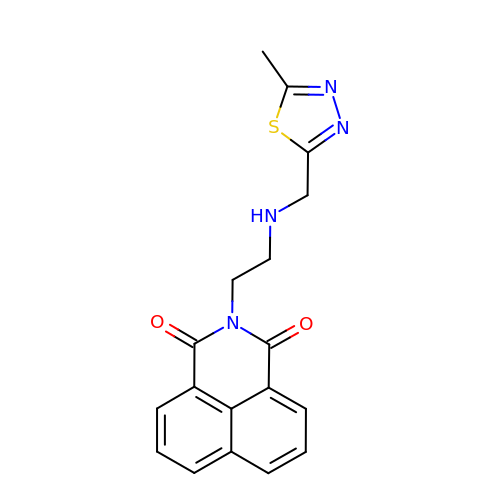2-(2-{[(5-methyl-1,3,4-thiadiazol-2-yl)methyl]amino}ethyl)-1H-benzo[de]isoquinoline-1,3(2H)-dione | C18 H16 N4 O2 S | YHPDOCZSFWEMOD-UHFFFAOYSA-N>[2x]MKKRAACLCFRSEREDEVLLVSSSRYP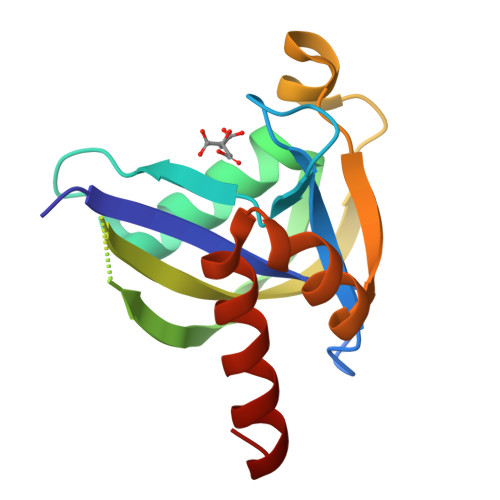DRWIVPGGGMEPEEEPGGAAVREVYEEAGVKGKLGRLLGVFEQNQDPEHRTYVYVLTVTELLEDWEDSVSIGRKREWFKVEDAIKVLQCHKPVHAEYLEKLKAHHHHHH> DVMTKEEQIFLLHRAQAQCEKRLKEVLQRPAGRPCLPEWDHIL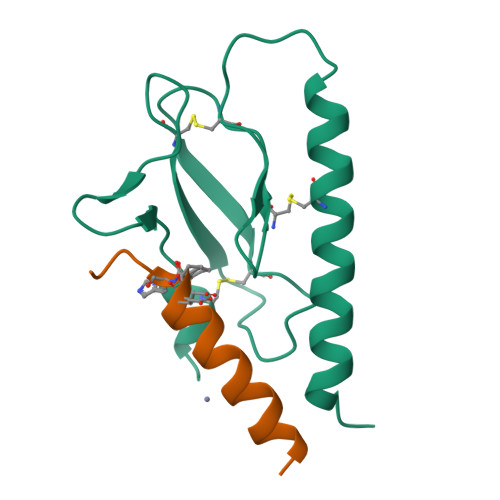CWPLGAPGEVVAVPCPDYIYDFNHKGHAYRRCDRNGSWELVPGHNRTWANYSECVKFL;> YQDLRRRFFLHHLIAEXHTAEIX> MGKSLPCDICKTVVTEAGNLLKDNATQEEILHYLEKTCEWIHDSSL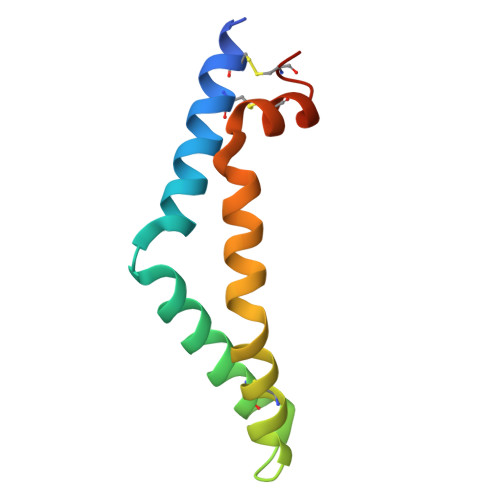SASCKEVVDSYLPVILDMIKGEMSNPGEVCSALNLCQSLQE>[2x]GSHMRDMIHNISYCLMVYGTEDEE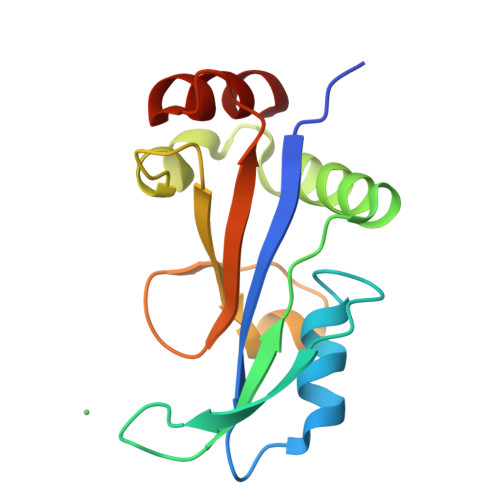KVIEALRNVIPGATPERESAEGYHGNPITVLRGRLDRRRALREFMEKFTEVFRGRMDELEDRFDENGNLFLRLDKQKALEGVWEPVRHGDAIHLKIKVEAYPAKREVAVENIRKILE CusB is a membrane fusion/adaptor protein (MFP) and CusC is an outer membrane (OM) protein belonging to the outer membrane factor (OMF family). Together, CusABC likely forms a protein complex spanning the inner membrane, periplasmic space and the outer membrane, analogous to the well-studied AcrAB-TolC multidrug efflux pump from E. coli and the MexAB-OprM multidrug efflux pump from Pseudomonas aeruginosa. Thus, the CusCFBA proteins form a tetrapartite system dedicated to the efflux of heavy metal ions from E. coli. Here we present the 2.3 Å X-ray crystal structure of CusC, the first structure of an outer membrane component of a heavy metal efflux pump.

There is one monomer of CusC (440 residues) within the asymmetric unit, with the biological trimer formed by the symmetry within the crystal. As is the case for the other OMF proteins, CusC is a cannon-shaped molecule, forming a ∼130 Å long α/β-barrel that is composed of three monomers. Each of the monomers contributes 4 β-strands to the 12-stranded β-barrel that resides within the OM, and 4 long α-helices to the periplasmic α-barrel. The CusC trimer forms a huge, continuous internal cavity with a cylindrical shape and a volume of ∼28,000 Å3 (∼90×20×20 Å), which is filled with water. By contrast, the interior of the entire barrel is strikingly electronegative. The channel is closed on this end by Van der Waals interactions between the Leu403 residues of the three monomers, analogous to the situation in OprM. In addition, an adjacent ring of negatively charged residues (Asp407) provides an additional layer of closure of the barrel on the periplasmic side. In our structure of CusC, density is clearly visible for three partial acyl chains attached to Cys1 of each CusC monomer; one single chain and another chain that is clearly branched. Thus, analogous to the E. coli Braun lipoprotein and many other bacterial lipoproteins, CusC is most likely triacylated at the N-terminal cysteine residue with N-acyl and S-diacylglycerol functions. In addition, despite the apparent specificity of CusC for small substrates, its extracellular opening is the largest observed for any OMF protein to date (∼30 Å diameter, measured as Cα-Cα distance).

> CSLAPDYQRPAMPVPQQFSLSQNGLVNAADNYQNAGWRTFFVDNQVKTLISEALVNNRDLRMATLKVQEARAQYRLTDADRYPQLNGEGSGSWSGNLKGNTATTREFSTGLNASFDLDFFGRLKNMSEAERQNYLATEEAQRAVHILLVSNVAQSYFNQQLAYAQLQIAEETLRNYQQSYAFVEKQLLTGSSNVLALEQARGVIESTRSDIAKRQGELAQANNALQLLLGSYGKLPQAQTVNSDSLQSVKLPAGLSSQILLQRPDIMEAEHALMAANANIGAARAAFFPSISLTSGISTASSDLSSLFNASSGMWNFIPKIEIPIFNAGRNQANLDIAEIRQQQSVVNYEQKIQNAFKEVADALALRQSLNDQISAQQRYLASLQITLQRARALYQHGAVSYLEVLDAERSLFATRQTLLDLNYARQVNEISLYTALGGGHHHHHH> P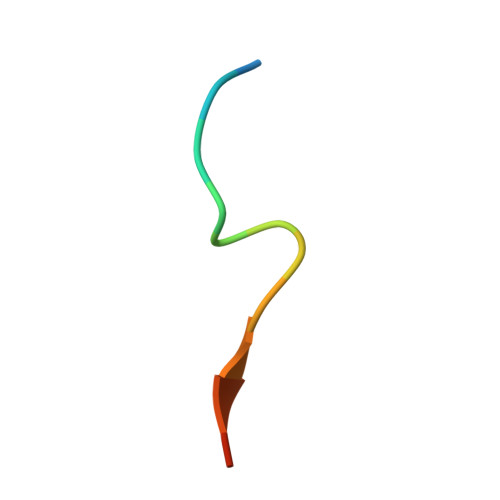KHTLDIFFKPLTH>[2x]MGHHHHHHHHHHMQSSVNEFLTPRHIDVQVVSQTRAKITLEPLERGFGHTLGNALRRILLSSMPGCAVVEAEIDGVLHEYSAIEGVQEDVIEILLNLKGLAIKLHGRDEVTLTLAKKGSGVVTAADIQLDHDVEIINGDHVIANLADNGALNMKLKVARGRGYEPADARQSDEDESRSIGRLQLDASFSPVRRVSYVVENARVEQRTNLDKLVLDLETNGTLDPEEAIRRAATILQQQLAAFVDLKGDSEPVVEEQEDEIDPILLRPVDDLELTVRSANCLKAENIYYIGDLIQRTEVELLKTPNLGKKSLTEIKDVLASRGLSLGMRLDNWPPASLKKDDKATA;> MGMAYSYTEKKRIRKDFSKLPDVMDVPYLLAIQLDSYREFLQAGATKEQFRDVGLHAAFKSVFPIISYSGNAALEYVGYRLGEPAFDVKECVLRGVTFAVPLRVKVRLIIFDRESSNKAIKDIKEQEVYMGEIPLMTENGTFIINGTERVIVSQLHRSPGVF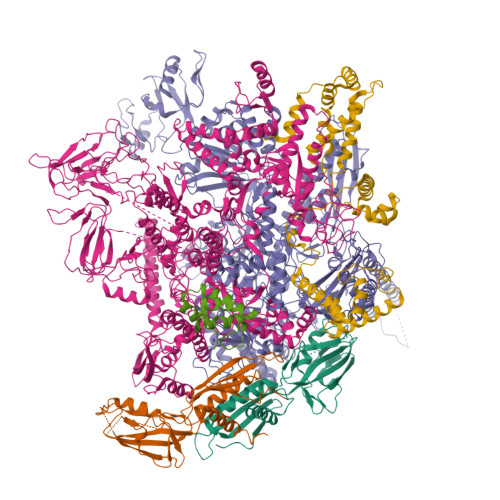FDHDRGKTHSSGKLLYSARIIPYRGSWLDFEFDPKDCVFVRIDRRRKLPASVLLRALGYSTEEILNAFYATNVFHIKGETLNLELVPQRLRGEVASIDIKDGSGKVIVEQGRRITARHINQLEKAGVSQLEVPFDYLIGRTIAKAIVHPATGEIIAECNTELTLDLLAKVAKAQVVRIETLYTNDIDCGPFISDTLKIDNTSNQLEALVEIYRMMRPGEPPTKEAAETLFGNLFFSAERYDLSAVGRMKFNRRIGRTEIEGPGVLSKEDIIDVLKTLVDIRNGKGIVDDIDHLGNRRVRCVGEMAENQFRVGLVRVERAVKERLSMAESEGLMPQDLINAKPVAAAIKEFFGSSQLSQFMDQNNPLSEITHKRRVSALGPGGLTRERAGFEVRDVHPTHYGRVCPIETPEGPNIGLINSLATYARTNKYGFLESPYRVVKDSLVTDEIVFLSAIEEADHVIAQASATLNEKGQLVDELVAVRHLNEFTVKAPEDVTLMDVSPKQVVSVAASLIPFLEHDDANRALMGSNMQRQAVPTLRADKPLVGTGMERNVARDSGVCVVARRGGVIDSVDASRVVVRVADDEVETGEAGVDIYNLTKYTRSNQNTCINQRPLVSKGDVVARGDILADGPSTDMGELALGQNMRVAFMPWNGFNFEDSICLSERVVQEDRFTTIHIQELTCVARDTKLGPEEITADIPNVGEAALNKLDEAGIVYVGAEVQAGDILVGKVTPKGETQLTPEEKLLRAIFGEKASDVKDTSLRVPTGTKGTVIDVQVFTRDGVERDSRALSIEKMQLDQIRKDLNEEFRIVEGATFERLRAALVGAKAEGGPALKKGTEITDDYLDGLERGQWFKLRMADDALNEQLEKAQAYISDRRQLLDDKFEDKKRKLQQGDDLAPGVLKIVKVYLAIKRRIQPGDKMAGRHGNKGVVSVIMPVEDMPHDANGTPVDIVLNPLGVPSRMNVGQILETHLGLAAKGLGEKINRMLEEQRKVAELRKFLHEIYNEIGGREENLDELGDNEILALAKNLRGGVPMATPVFDGAKEREIKAMLKLADLPESGQMRLFDGRTGNQFERPTTVGYMYMLKLNHLVDDKMHARSTGSYSLVTQQPLGGKAQFGGQRFGEMEVWALEAYGAAYTLQEMLTVKSDDVNGRTKMYKNIVDGDHRMEAGMPESFNVLIKEIRSLGIDIELETE;> MLKDLLNLLKNQGQIEEFDAIRIGLASPEMIRSWSFGEVKKPETINYRTFKPERDGLFCAKIFGPVKDYECLCGKYKRLKHRGVICEKCGVEVALAKVRRERMGHIELASPVAHIWFLKSLPSRIGLLLDMTLRDIERVLYFESYVVIDPGMTTLEKGQLLNDEQYFEALEEFGDDFDARMGAEAVHELLNAIDLEHEIGRLREEIPQTNSETKIKKLSKRLKLMEAFQGSGNKPEWMVLTVLPVLPPDLRPLVPLDGGRFATSDLNDLYRRVINRNNRLKRLLDLAAPDIIVRNEKRMLQEAVDALLDNGRRGRAITGSNKRPLKSLADMIKGKQGRFRQNLLGKRVDYSGRSVITVGPTLRLHQCGLPKKMALELFKPFIFGKLEGRGMATTIKAAKKMVERELPEVWDVLAEVIREHPVLLNRAPTLHRLGIQAFEPVLIEGKAIQLHPLVCAAYNADFDGDQMAVHVPLTLEAQLEARALMMSTNNILSPANGEPIIVPSQDVVMGLYYMTREAINAKGEGMAFADLQEVDRAYRSGQASLHARVKVRINEKIKGEDGQLTANTRIVDTTVGRALLFQVVPAGLPFDVVNQSMKKKAISKLINHCYRVVGLKDTVIFADQLMYTGFAYSTISGVSIGVNDFVIPDEKARIINAATDEVKEIESQYASGLVTQGEKYNKVIDLWSKANDEVSKAMMANLSKEKVVDREGKEVDQESFNSMYMMADSGARGSAAQIRQLAGMRGLMAKPDGSIIETPITANFREGLNVLQYFISTHGARKGLADTALKTANSGYLTRRLVDVAQDLVVTEIDCGTEHGLLMSPHIEGGDVVEPLGERVLGRVIARDVFKPGSDEVIVPAGTLIDEKWVDFLEVMSVDEVVVRSPITCETRHGICAMCYGRDLARGHRVNIGEAVGVIAAQSIGEPGTQLTMRTFHIGGAASRTSAADNVQVKNGGTIRLHNLKHVVRADGALVAVSRSGELAVADDFGRERERYKLPYGAVISVKEGDKVDPGAIVAKWDPHTHPIVTEVDGTVAFVGMEEGITVKRQTDELTGLTNIEVMDPKDRPAAGKDIRPAVKLIDAAGKDLLLPGTDVPAQYFLPANALVNLTDGAKVSIGDVVARIPQETSKTRDITGGLPRVADLFEARRPKEPSILAEISGTISFGKETKGKRRLVITPNDGSDPYEELIPKWRHLNVFEGEQVNRGEVISDGPSNPHDILRLLGVSSLAKYIVNEIQDVYRLQGVKINDKHIETILRQMLRKVEVSESGDSSFIKGDQVELTQVLEENEQLGTEDKFPAKYERVLLGITKASLSTESFISAASFQETTRVLTEAAVTGKRDFLRGLKENVVVGRLIPAGTGLAYHSERKRQRDLGKPQRVSASEAEAALTEALNSSGNGSGSWSHPQFEK;> MARVTVEDCLDNVDNRFELVMLATKRARQLATGGKEPKVAWENDKPTVVALREIASGLVDENVVQQEDIVEDEPLFAAFDDEANTEAL;> GAMGMALKKEGPEFDHDDEVLLLEPGIMLDESSADEQPSPRATPKATTSFSSKQHKHIDYTRALDATQLYLNEIGFSPLLTPEEEVHFARLAQKGDPAGRKRMIESNLRLVVKIARRYVNRGLSLLDLIEEGNLGLIRAVEKFDPERGFRFSTYATWWIRQTIERAIMNQTRTIRLPIHVVKELNVYLRAARELTHKLDHEPSPEEIANLLEKPVAEVKRMLGLNERVTSVDVSLGPDSDKTLLDTLTDDRPTDPCELLQDDDLSESIDQWLTELTDKQREVVIRRFGLRGHESSTLEEVGQEIGLTRERVRQIQVEALKRLREILEKNGLSSDALFQ>[12x]GSGDSGSPGEKFYWRAKSQMCEVKGWVPTHRGFPWGPELPGDLILSRRAYVSCDLTSCFKFFIAYGLSANQHLLNTSMEWEESLYKTPIGSASTLSTSEMILPGRSSSACFDGLKWTVLVANGRDRNSFI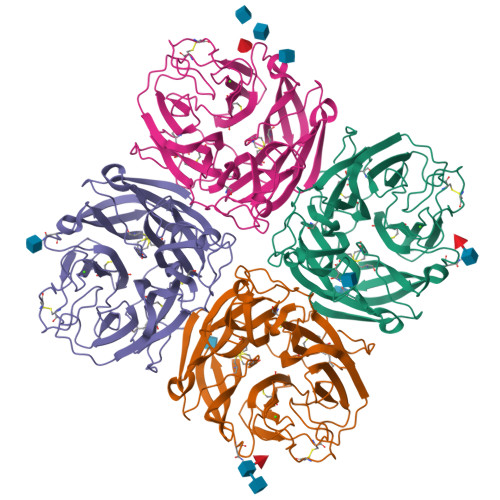MIKYGEEVTDTFSASRGGPLRLPNSECICIEGSCFVIVSDGPNVNQSVHRIYELQNGTVQRWKQLNTTGINFEYSTCYTINNLIKCTGTNLWNDAKRPLLRFTKELNYQIVEPCNGAPTDFPRGGLTTPSCKMAQEKGEGGIQGFILDEKPAWTSKTKAESSQNGFVLEQIPNGIESEGTVSLSYELFSNKRTGRSGFFQPKGDLISGCQRICFWLEIEDQTVGLGMIQELSTFCGINSPVQNINWDS> MGSSHH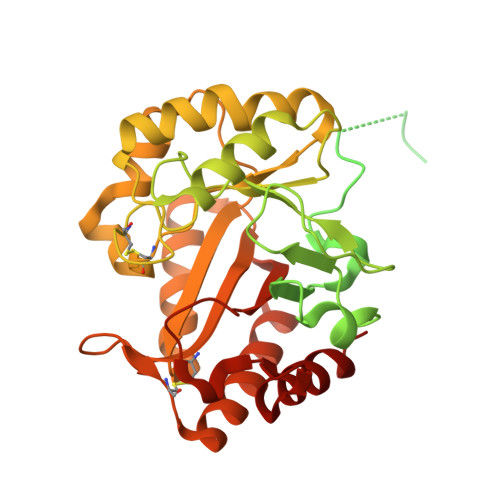HHHHSSGLVPAGSHMSSLHPNAAAHRRQDITHERVNSAVERRETLAQSQPRALSEKPNKRKITRRGGRSCRARNSTATASDSATASTPSQNSTAALPDSTDSYVASAVSSGAESSSSTQAPVENTSSSSEDVAATTSSIENIAALQQPSSSSSAEDSSTAANSTSVASAAATSSAAATSSSSSSSNSTGSYTPNGIKAGVSGDDPLSFLQGHIGWYYDWNATPSGSASGASAVNMLWGAGTVDSTDASRLSAFKALTTAPQYIIGFEEPDCSTPGSSNIAVADAASLWDSTIAPWKDQGSILISPSMCHQAAEEYTKWLSAFSSQISTSWDITNLHINKNSMDGVKTDIDYYYNTYGKPIWVTEFACVDDSTDFVPCTDQSEINTFINDIVALFESDDRVQAYAYSTGEGLSPEWDMISNGALTESGQTYLTAISQYH>[3x]PIELLPETPSQTAGPYVHIGLALEAAGNPTRDQEIWNRLAKPDAPGEHILLLGQVYDGNGHLVRDSFLEVWQADANGEYQDAYNLENAFNSFGRTATTFDAGEWTLHTVKPGVVNNAAGVPMAPHINISLFARGINIHLHTRLYFDDEAQANAKCPVLNLIEQPQRRETLIAKRCEVDGKTAYRFDIRIQGEGETVFFDF;>[3x]PAQDNSRFVIRDRNWHPKALTPDYKTSIARSPRQA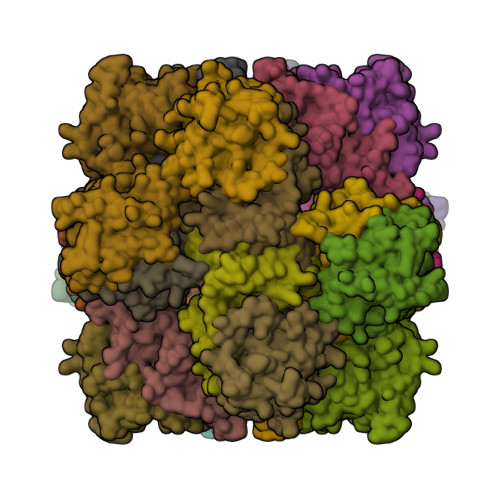LVSIPQSISETTGPNFSHLGFGAHDHDLLLNFNNGGLPIGERIIVAGRVVDQYGKPVPNTLVEMWQANAGGRYRHKNDRYLAPLDPNFGGVGRCLTDSDGYYSFRTIKPGPYPWRNGPNDWRPAHIYFGISGPSIATKLITQLYFEGDPLIPMCPIVKSIANPEAVQQLIAKLDMNNANPMDCLAYRFDIVLRGQRKTHFENC> MTRVVYKVPEEQPPNTLIGSLAADY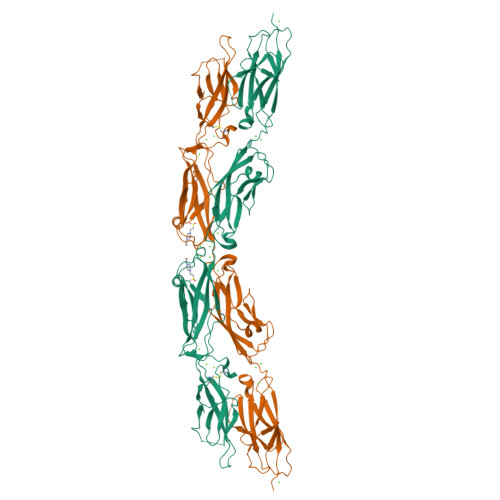GFPDVGHLYKLEVGAPYLRVDGKTGDIFTTETSIDREGLRECQNQLPGDPCILEFEVSITDLVQNGSPRLLEGQIEVQDINDNTPNFASPVITLAIPENTNIGSLFPIPLASDRDAGPNGVASYELQAGPEAQELFGLQVAEDQEEKQPQLIVMGNLDRERWDSYDLTIKVQDGGSPPRASSALLRVTVLDTNDNAPKFERPSYEAELSENSPIGHSVIQVKANDSDQGANAEIEYTFHQAPEVVRRLLRLDRNTGLITVQGPVDREDLSTLRFSVLAKDRGTNPKSARAQVVVTVKDMNDNAPTIEIRGIGLVTHQDGMANISEDVAEETAVALVQVSDRDEGENAAVTCVVAGDVPFQLRQASETGSDSKKKYFLQTTTPLDYEKVKDYTIEIVAVDSGNPPLSSTNSLKVQVVDVNDNALEHHHHHH> QSACTLQSETHPPLTWQKCSSGGTCTQQTGSVVIDANWRWTHATNSSTNCYDGNTWSSTLCPDNETCAKNCCLDGAAYASTYGVTTSGNSLSIGFVTQSAQKNVGARLYLMASDTTYQEFTLLGNEFSFDVDVSQLPCGLNGALYFVSMDADGGVSKYPTNTAGAKYGTGYCDSQCPRDLKFINGQANVEGWEPSSNNANTGIGGHGSCCSEMDIWQANSISEALTPHPCTTVGQEICEGDGCGGTYSDNRYGGTCDPDGCDWNPYRLGNTSFYGPGSSFTLDTTKKLTVVTQFETSGAINRYYVQNGVTFQQPNAELGSYSGNELNDDYCTAEEAEFGGSSFSDKGGLTQFKKATSGGMVLVMSLWDDY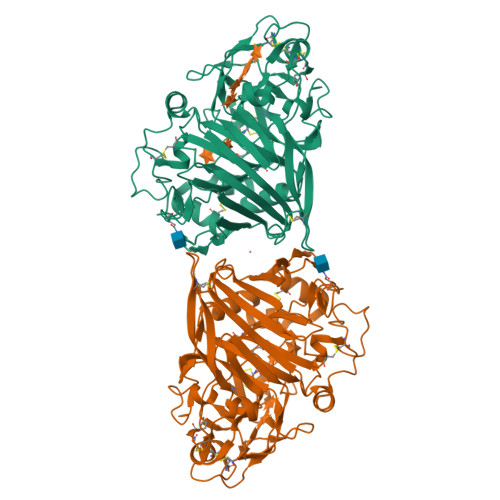YANMLWLDSTYPTNETSSTPGAVRGSCSTSSGVPAQVESQSPNAKVTFSNIKFGPIGSTGNPSG>[2x]MSALFEPYTLKDVTLRNRIAIPPMCQYMAEDGLINDWHQVHYASMARGGAGLLVVEATAVAPEGR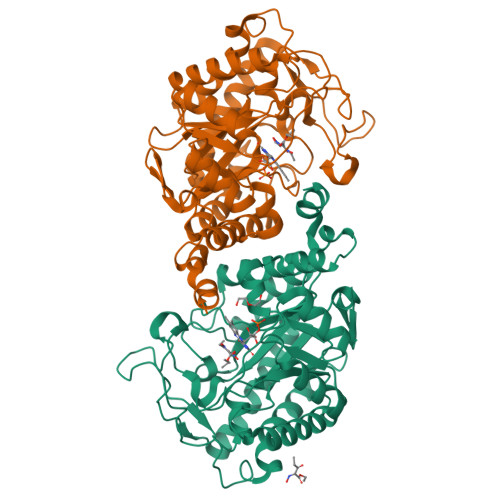ITPGCAGIWSDAHAQAFVPVVQAIKAAGSVPGIQIAHAGRKASANRPWEGDDHIGADDARGWETIAPSAIAFGAHLPNVPRAMTLDDIARVKQDFVDAARRARDAGFEWIELHFAHGFLGQSFFSEHSNKRTDAYGGSFDNRSRFLLETLAAVREVWPENLPLTARFGVLEYDGRDEQTLEESIELARRFKAGGLDLLSVSVGFTIPETNIPWGPAFMGPIAERVRREAKLPVTSAWGFGTPQLAEAALQANQLDLVSVGRAHLADPHWAYFAAKELGVEKASWTLPAPYAHWLERYRLEHHHHHH> MLKHEGPPAEKPLEELSASTSGVPGLSSLQSDPAGCV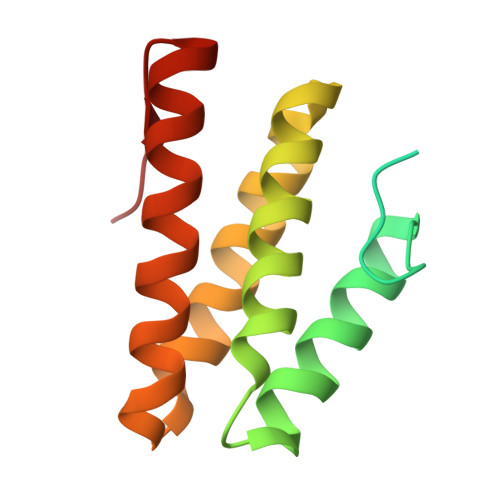RPPAPNLAGAVEFNDVKTLLREWITTISDPMEEDILQVVKYCTDLIEEKDLEKLDLVIKYMKRLMQQSVESVWNMAFDFILDNVQVVLQQTYGSTLKVT>MKEVIAVKEITRFKTRTEEFSPYAWCKRMLENDPVSYHEGTDTWNVFKYEDVKRVLSDYKHFSSVRKRTTISVGTDSEEGSVPEKIQITESDPPDHRKRRSLLAAAFTPRSLQNWEPRIQEIADELIGQMDGGTEIDIVASLASPLPIIVMADLMGVPSKDRLLFKKWVDTLFLPFDREKQEEVDKLKQVAAKEYYQYLYPIVVQKRLNPADDIISDLLKSEVDGEMFTDDEVVRTTMLILGAGVETTSHLLANSFYSLLYDDKEVYQELHENLDLVPQAVEEMLRFRFNLIKLDRTVKEDNDLLGVELKEGDSVVVWMS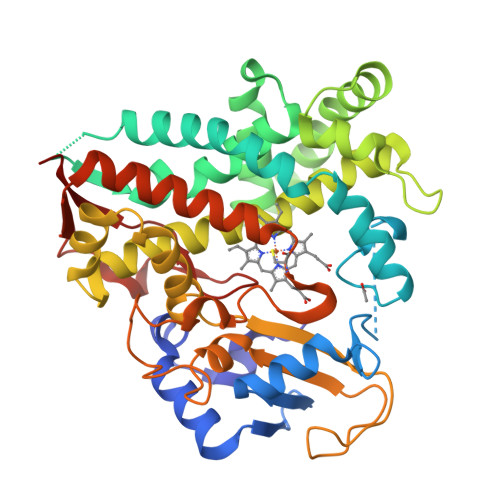AANMDEEMFEDPFTLNIHRPNNKKHLTFGNGPHFCLGAPLARLEAKIALTAFLKKFKHIEAVPSFQLEENLTDSATGQTLTSLPLKASRM[2x]> MFRPTTAIADSFKEHYHRVHLPRRLALQRYARQQSLRNAAKGNVKAEEVPYKYNRWW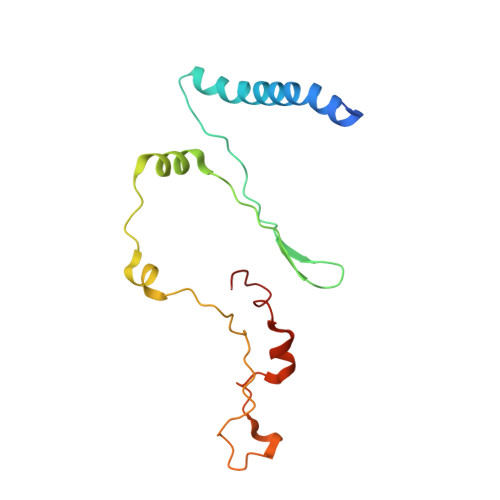VNEEHEFVHQYAFVEDPEVTKAKRETLPPVTRENIWKEPQQTFFLPFAPYVRVVDYPKDPDAKFLKPVNIPRWKDYMQRTKPVIPRTWY>[2x]MKKLGTLLVLFLSAIILVACASGKKDTTSGQKLKVVATNSIIADITKNIAGDKIDLHSIVPIGQDPHEYEPLPEDVKKTSEADLIFYNGI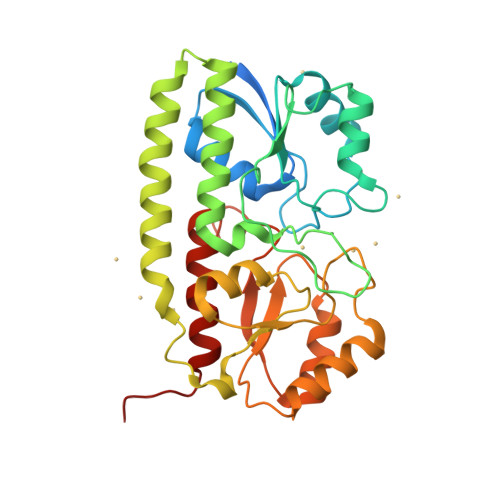NLETGGNAWFTKLVENAKKTENKDYFAVSDGVDVIYLEGQNEKGKEDPHAWLNLENGIIFAKNIAKQLSAKDPNNKEFYEKNLKEYTDKLDKLDKESKDKFNKIPAEKKLIVTSEGAFKYFSKAYGVPSAYIWEINTEEEGTPEQIKTLVEKLRQTKVPSLFVESSVDDRPMKTVSQDTNIPIYAQIFTDSIAEQGKEGDSYYSMMKYNLDKIAEGLAKGNLYF> GSHMRLGAQSIQPTANLDRTDDLVYLNVMELVRAVLELKNELAQLPPEGYVVVVKNVGLTLRKLIGSVDDLLPSLPSS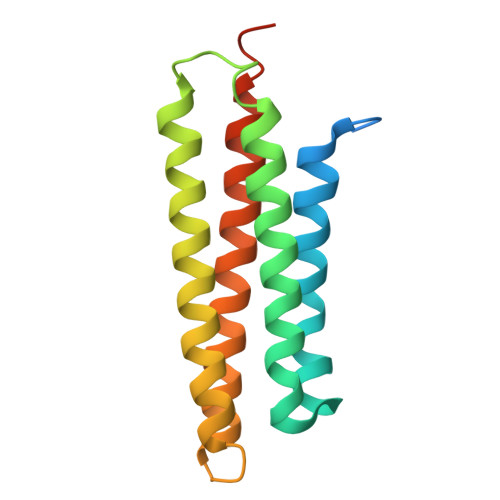SRTEIEGTQKLLNKDLAELINKMRLAQQNAVTSLSEECKRQMLTASHTLAVDAKNLLDAVDQAKVLANLAHPPAE> RSLPSCKEDEYPVGSECCPKCSPGYRVKEACGELTGTVCEPCPPGTYIAHLNGLSKCLQCQMCDPAMGLRASRNCSRTENAVCGCSPGHFCI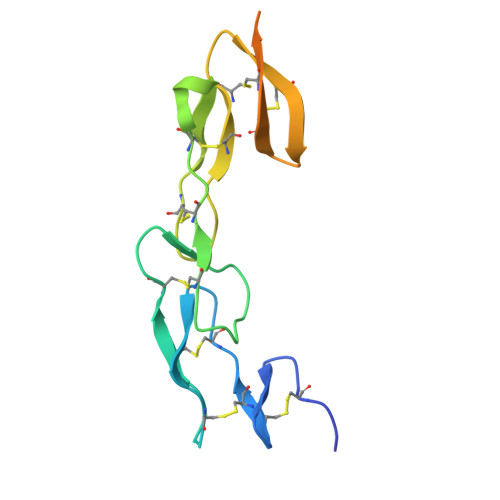VQDGDHCAACRAYATSSPGQRVQKGGTESQDTLCTGHHHHHH>MTAPTVPVALVTGAAKRLGSGIAEGLHAEGYAVCLHYHRSAAEANTLAATLNARRPNSAIPVQADLSNVAKAPAGGADGAAPVTLFKRCADLVAACYTHWGRCDVLVNNASSFYPTPLLRKDEDGHVPCVGDREAMEAAAADLFGSNAMAPYFLIKAFAHRVADTPAEQRGTNYSIVNMVDAMTSQPLLGYTIYTMAKGALEGLTRSAALELAPLQIRVNGVGPGLSVLADDMPPAVREDYRSKVPLYQRDSSAAEVSDVVIFLCSSKAKYVTG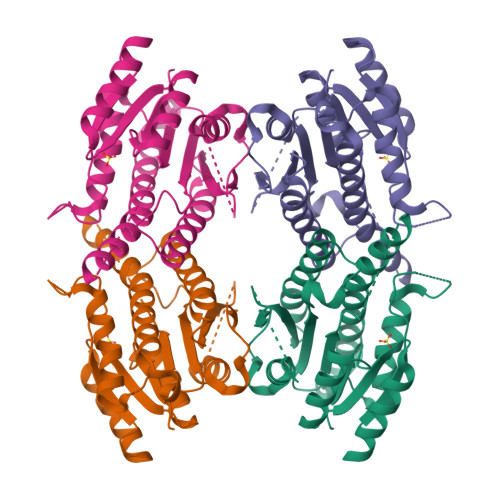TCVKVDGGYSLTRA[2x]>[4x]MSNLSLDFSDNTFQPLAARMRPENLAQYIGQQHLLAAGKPLPRAIEAGHLHSMILWGPPGTGKTTLAEVIARYANADVERISAVTSGVKEIREAIERARQNRNAGRRTILFVDEVHRFNKSQQDAFLPHIEDGTITFIGATTENPSFELNSALLSRARVYLLKSLSTEDIEQVLTQAMEDKTRGYGGQDIVLPDETRRAIAELVNGDARRALNTLEMMADMAEVDDSGKRVLKPELLTEIAGERSARF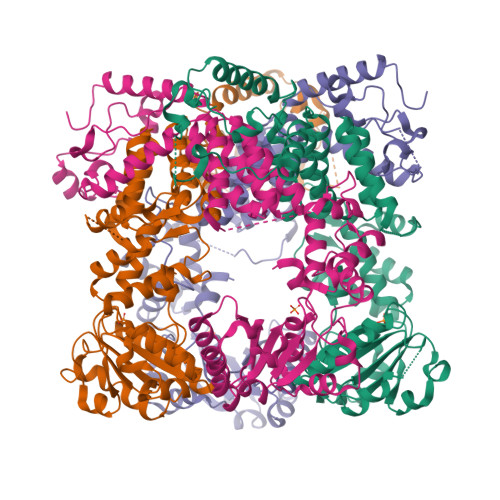DNKGDRFYDLISALHKSVRGSAPDAALYWYARIITAGGDPLYVARRCLAIASEDVGNADPRAMQVAIAAWDCFTRVGPAEGERAIAQAIVYLACAPKSNAVYTAFKAALADARERPDYDVPVHLRNAPTKLMKEMGYGQEYRYAHDEANAYAAGEVYFPPEIAQTRYYFPTNRGLEGKIGEKLAWLAEQDQNSPIKRYR>AQVINTFDGVADYLQTYHKLPDNYITKSEAQALGWVASKGNLADVAPGKSIGGDIFSNREGKLPGKSGRTWREADINYTSGF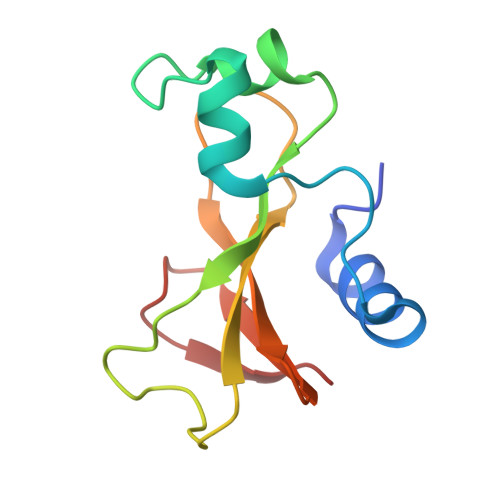RNSDRILYASDWLIYKTTDHYQTFTKIR[3x]> MRGSHHHHHHIQESRLDRILESGVLRVATTGDYKPFSYRTEEGGYAGFDVDMAQRLAESLGAKLVVVPTSWPNLMRDFADDRFDIAMSGISINLERQRQAYFS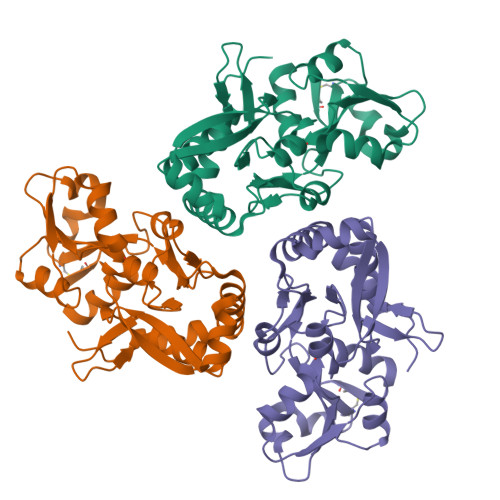IPYLRDGKTPITLCSEEARFQTLEQIDQPGVTAIVNPGGTNEKFARANLKKARILVHPDNVTIFQQIVDGKADLMMTDAIEARLQSRLHPELCAVHPQQPFDFAEKAYLLPRDEAFKRYVDQWLHIAEQSGLLRQRMEHWLEYRWPTAHGKL GLYCOCHOLIC ACID | C26 H43 N O6 | 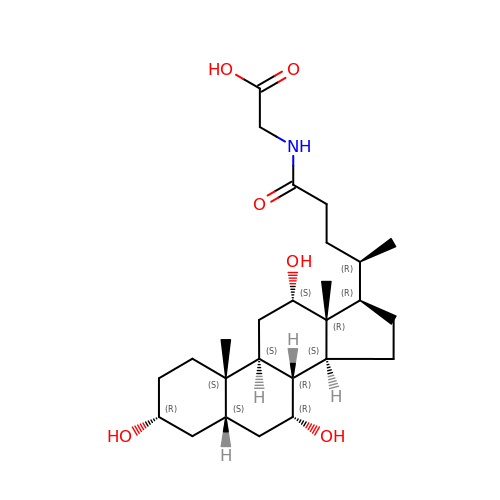RFDAIACWWDREDC-FRVQLJSFSA-N> GSMTNFQTWLDSADIPVQQNGQWIDLETGIAYDPSYNYAANTRRAS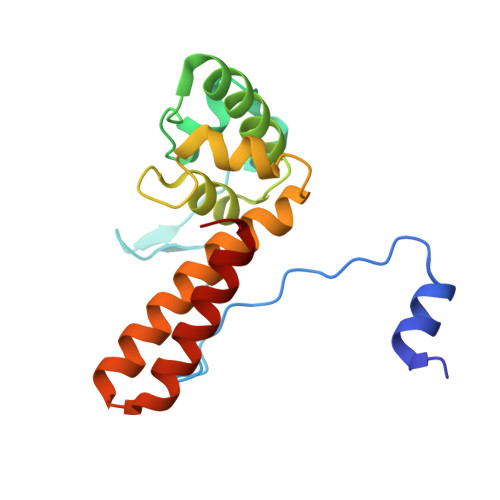LSPRGIDARAVAKTFGGRALTGTARQKEWAEKIRAEKVQQMNQDQAEMACDPSGLLTAAKFWIENRNDSAQEIAGFVMQQKALLAQHRSAKAAGQADKVAKIAAEYNALTARWGF>MAGLYTTYQLLEVQRKLKTLPAFFLQWFPRQINFQEDMIAFDKVIQDVTRVAPFVAPNVQGRVIKESGYNTKTFKPAYVKPKHVIDPNMIIPRQPGEALGTGTLSIAQRRDRVIAYLLMKHRAMHENTWEWMAAQAAQYGYVDVQGQDYPLVRVDFGRDAALTMTTDWTAAGVTLMDMIADLRDGQRLVSDKSMSGTVIRDYVFGGDAWDQFVKVGGKELWGKDGLMDSTIRGSETNVTRLWDDVEGVQYMGELVGANGAGRMRIWVNTQKYRDQNDQEQFLMKQKAVMGISSAIEGVRCFGAILDKGAGYQALDYFPKMWDQEDPSVEYLMSQGAPLMVPADPNASFLLTVMS[7x];>MNLLTMMAATSLPNYLAGNGDLGSWEPTQIFAGEADIVTEGGAAGADIEIYQVIAKNAAGAMVPHDPTATTGTSPDEVPAPQSVAIGIAAQPAKSGQNVPYYIGGVFNHAALGWHASLDTLAKRQAVFDRTNIHIGNLY[7x]

Here we have determined by cryo-electron microscopy (cryo-EM) structures of the head and tail components of YSD1, a phage infecting Salmonella Typhi. We investigated the structure of the recently characterised phage YSD1 as an example of flagellotropic χ-like phages and more generally phages with long, non-contractile tails. Samples of YSD1 imaged by EM showed characteristic features of siphoviruses: an icosahedral capsid and a flexible tail tube of ~220 nm in length. Cryo-EM analysis of YSD1 allowed structure determination of the head and tail components at resolutions of 3.8 Å and 3.5 Å, respectively, and the generation of de novo models for the major capsid (YSD1_17), auxiliary protein (YSD1_16) and tail-tube protein (YSD1_22).

YSD1 has an icosahedral head organised with a T = 7 laevo symmetry. The mature head contains 415 major capsid proteins arranged in hexon and penton capsomers, forming a shell that is remarkably thin for its ~650 Å diameter. This shell is further decorated by trimers of the auxiliary protein located at each threefold or pseudo threefold position. First, a clamp formed by two loops, C1 and C2 immobilises the E-loop around the threefold axes. Second, trimers of the auxiliary protein dock at the threefold axes over the clamp and E-loop locking in place this critical capsomer interface. In both YSD1 and λ, the N-terminus of the auxiliary protein staples neighbouring capsomers by interactions around the twofold axis augmenting the major capsid β-sheet of the E-loop/N-terminal arm. However, in the flagellotropic χ-like phages, an additional hook-like structure formed by an N-terminal extension connects trimers of the auxiliary proteins. This interaction mediates the formation of an external protein network that braces the inner capsid shell.> DIPQPIRGDKGATVKIPRNIERDRQNPDMLVPPETDHGTVSNMKFSFSDTHNRLEK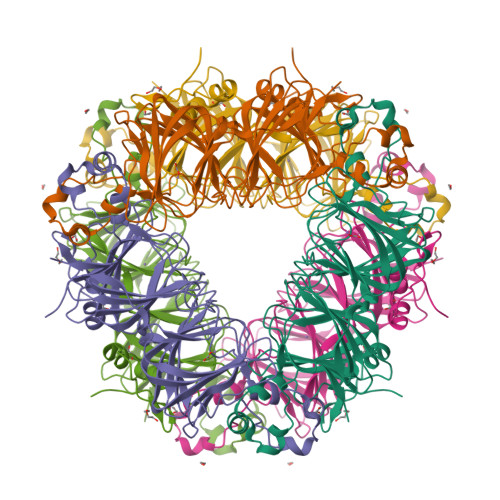GGYAREVTVRELPISENLASVNMRLKPGAIRELHWHKEAEWAYMIYGSARVTIVDEKGRSFIDDVGEGDLWYFPSGLPHSIQALEEGAEFLLVFDDGSFSENSVFQLTDWLAHTPKEVIAANFGVTKEEISNLPGKEKYIFENQLPGSLKDDIVEGPNGEVPYPFTYRLLEQEPIESEGGKVYIADSTNFKVSKTIASALVTVEPGAMRELHWHPNTHEWQYYISGKARMTVFASDGHARTFNYQAGDVGYVPFAMGHYVENIGDEPLVFLEIFKDDHYADVSLNQWLAMLPETFVQAHLDLGKDFTDVLSKEKHPVVKKK>[2x]GMPNYKLTYFN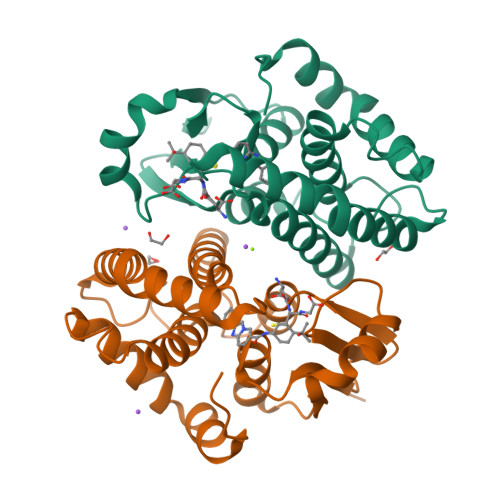MRGRAEIIRYIFAYLDIQYEDHRIEQADWPEIKSTLPFGKIPILEVDGLTLHQSLAIARYLTKNTDLAGNTEMEQCHVDAIVDTLDDFMSCFPWAEKKQDVKEQMFNELLTYNAPHLMQDLDTYLGGREWLIGNSVTWADFYWEICSTTLLVFKPDLLDNHPRLVTLRKKVQAIPAVANWIKRRPQTKL(2E,5R)-5-(2-cyclohexylethyl)-2-imino-3-methyl-5-{[(1S,3R)-3-(quinolin-2-ylamino)cyclohexyl]methyl}imidazolidin-4-one 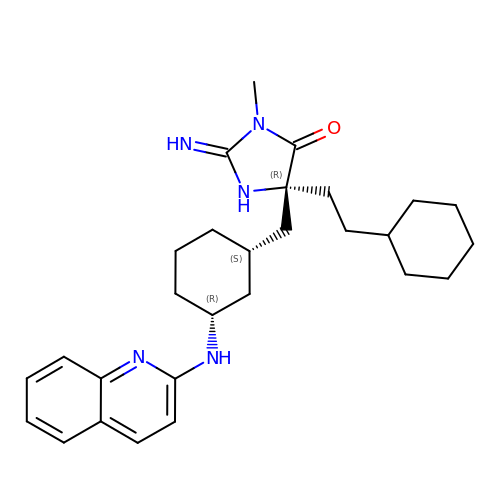| C28 H39 N5 O | XBQKWFZOPAEITA-TWLCBMPQSA-N>[6x]MTQMLTRPDVDLVNGMFYADGGAREAYRWMRANEPVFRDRNGL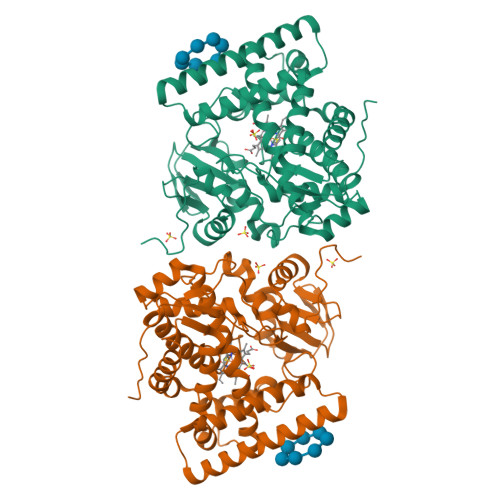AAATTYQAVLDAERNPELFSSTGGIRPDQPGMPYMIDMDDPQHLLRRKLVNAGFTRKRVMDKVDSIGRLCDTLIDAVCERGECDFVRDIAAPLPMAVIGDMLGVLPTERDMLLKWSDDLVCGLSSHVDEAAIQKLMDTFAAYTEFTKDVITKRRAEPTDDLFSVLVNSEVEGQRMSDDEIVFETLLILIGGDETTRHTLSGGTEQLLRHRDQWDALVADVDLLPGAIEEMLRWTSPVKNMCRTLTADTVFHGTELRAGEKIMLMFESANFDESVFGDPDNFRIDRNPNSHVAFGFGTHFCLGNQLARLELRLMTERVLRRLPDLRLADDAPVPLRPANFVSGPESMPVVFTPSAPVLAHHHHHH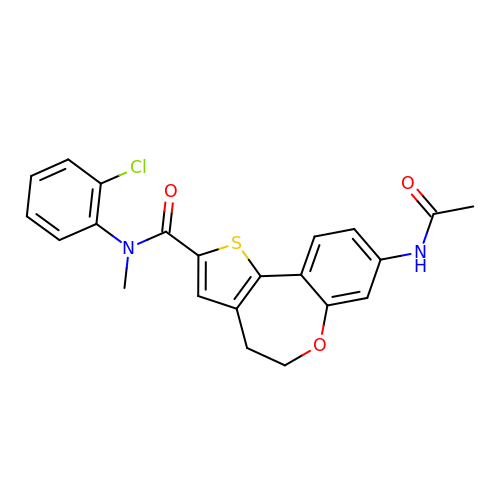8-(acetylamino)-N-(2-chlorophenyl)-N-methyl-4,5-dihydrothieno[3,2-d][1]benzoxepine-2-carboxamide | C22 H19 Cl N2 O3 S | RTUHEKLMDKJAQG-UHFFFAOYSA-N>GGGGCTCC[2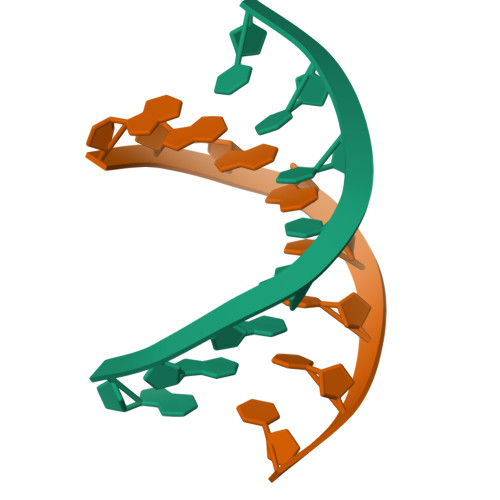x]>QNVGTQAAEEPLNLPISVCTAPGNCQTEADAVVLDSNWRWAHTTTGYTNCYTGNLWDTTLCPTPETCTTNCAIDGVPLADWSGTYGGSVTGNKFNLKFVTVGPYSTNIGARTFLLDSTKTRYRMFQLLNREFTYDVDVSSLDCGLNGALYFVSMDADGGAAKYPTNKGGAKYGTGYCDAQCPHDVKWINGLANSKDWTPIPGDANSGKGYYGNCCAELDIWEANKQSQAFTTHPCTPNDQTRCEGVVCGDNDSGDRYNGMCDKDGCDFASYRMNDHTFYGPGSTFKLDSTKPFTVVSQFITTDGTDNGDFKEFRRFYV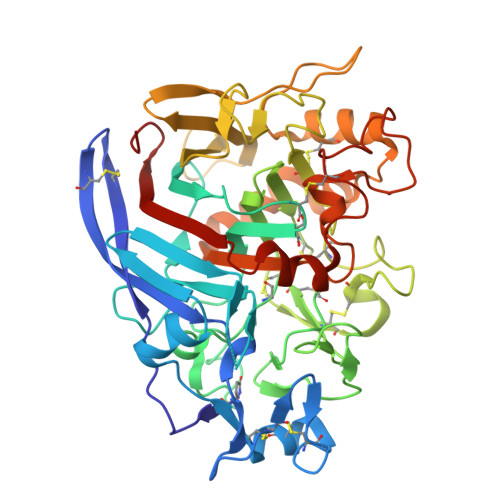QNGVRIENSKVNFPGITAYDSITDEMCAATKGLFGDLDDHKNKGGMKQMGEAMRKGMALVMSIWDDHDVNMLWLDSNYPPTGNPSTPGVARGPCPTTSGVPSEVEVTQANAVVSFGNIKFGPIGSTV[2x]> AAIVAGPKQNCEPDLMPYARPFAVGKRTCSGIVGLPSGSDPAFSQPKSVLDAGLTCQGASPSSVSKPILLVPGTGTTGPQSFDSNWIPLSAQLGYTPCWISPPPFMLNDTQVNTEYMVNAITTLYAGSGNNKLPVLTWSQGGLVAQWGLTFFPSIRSKVD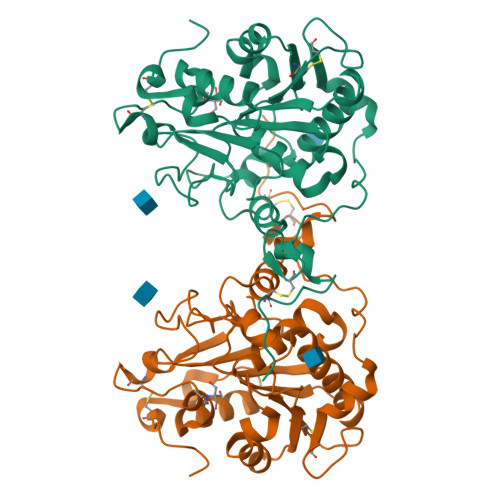RLMAFAPDYKGTVLAGPLDALAVSAPSVWQQTTGSALTTALRNAGGLTQIVPTTNLYSATDEIVQPQVSNSPLDSSYLFNGKNVQAQAVCGPLFVIDHAGSLTSQFSYVVGRSALRSTTGQARSADYGITDCNPLPANDLTPEQKVAAAALLAPAA> MKEFYLTVEQIGDSIFERYIDSNGRERTREVEYKPSLFAHCPESQATKYFDIYGKPCTRKLFANMRDASQWIKRMEDIGLEALGMDDFKLAYLSDTYNYEIKYDHTKIRVANFDIEVTSPDGFPEPSQAKHPIDAITHYDSIDDRFYVFDLLNSPYGNVEEWSIEIAAKLQEQGGDEVPSEIIDKIIYMPFDNEKELLMEYLNFWQQKTPVILTGWNVESFAIPYVYNRIKNIFGESTAKRLSPHRKTRVKVIENMYGSREIITLFGISVLDYIDLYKKFSFTNQPSYSLDYISEFELNVGKLKYDGPISKLRESNHQRYISYNIIAVYRVLQIDAKRQFINLSLDMGYYAKIQIQSVFSPIKTWDAIIFNSLKEQNKVIPQGRSHPVQPYPGAFVKEPIPNRYKYVMSFDLTSLYPSIIRQVNISPETIAGTFKVAPLHDYINAVAERPSDVYSCSPNGMMYYKDRDGVVPTEITKVFNQRKEHKGYMLAAQRNGEIIKEALHNPNLSVDEPLDVDYRFDFSDEIK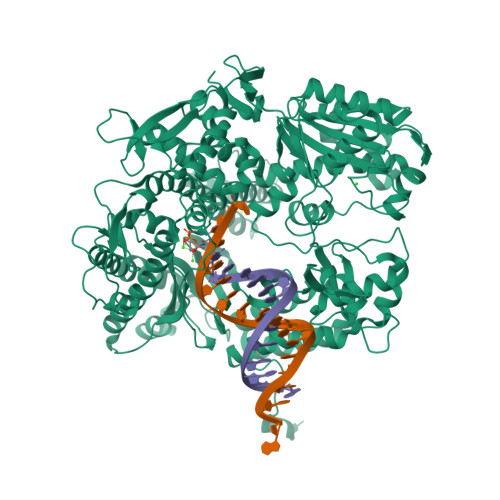EKIKKLSAKSLNEMLFRAQRTEVAGMTAQINRKLLINSLYGALGNVWFRYYDLRNATAITTFGQMALQWIERKVNEYLNEVCGTEGEAFVLYGDTDSIYVSADKIIDKVGESKFRDTNHWVDFLDKFARERMEPAIDRGFREMCEYMNNKQHLMFMDREAIAGPPLGSKGIGGFWTGKKRYALNVWDMEGTRYAEPKLKIMGLETQKSSTPKAVQKALKECIRRMLQEGEESLQEYFKEFEKEFRQLNYISIASVSSANNIAKYDVGGFPGPKCPFHIRGILTYNRAIKGNIDAPQVVEGEKVYVLPLREGNPFGDKCIAWPSGTEITDLIKDDVLHWMDYTVLLEKTFIKPLEGFTSAAKLDYEKKASLFDMFD> MLDSLKSQFQPSFPRLASGHYVHFLMLRHSQSFPVFQTDGVLNTTRTQAGLLEKTDQLSRLVMFKRKQTTPERLAGRELLRNLGLTSADKSAKNLCEYNGEGSCKQCPDCILYGFAIGDSGSERSKVYSDSAFSLGAYEQSHRSFTFNAPFEGGTMSEAGVMRSAINELDHILPEVTFPTVESLRDATYEGFIYVLGNLLRTKRYGAQESRTGTMKNHLVGIVFADGEIFSNLHL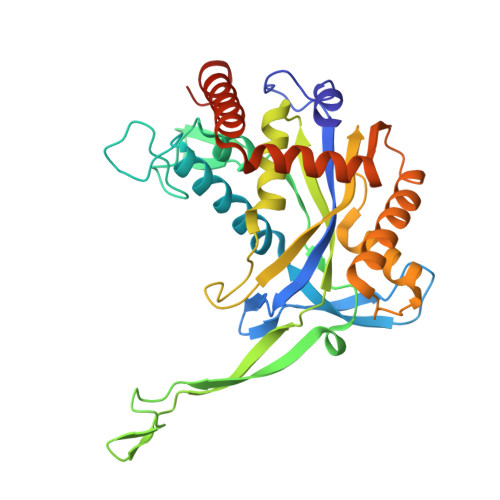TQALYDQMGGELNKPISELCETAATVAQDLLNKEPVRKSELIFGAHLDTLLQEVNDIYQNDAELTKLLGSLYQQTQDYATEFGALSGGKKKAKS>[12x]MERNHWNEKSSGAKRSRERDLTLSTIRSILAADERLRIKASSYLGVGRGVDDEAVIDIFPTGQTMSFLRLLHGFLGTCRGQSMHQVLRDPCVLRKQLLYGVCKTLFDTITVRRVAEEWKLHAALFPYRALDEEDLEQYLLVWSASLRQSVQTGVLGALRDILYQYADNDDYGLYVDWCVTVGLVPLLDVKTKPSEAAERAQFVRAAVQRATETHPLAQDLLQANLALLLQVAERLGAVRVANAPEVRVFKKVRSERLEAQLRGKHIRLYVAAEPLAYERDKLLFTTPVAHLHEEILRYDGLCRHQKICQLLNTFPVKVVTASRHELNCKKLVEMMEQHDRGSDAKKSIM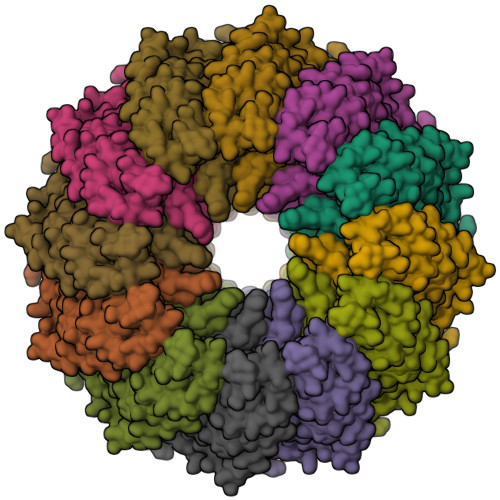KFLLNVSDSKSRIGIEDSVESFLQDLTPSLVDQNRLLPARGPGGPGVVGPGGAVVGGPAGHVGLLPPPPGPAAPERDIRDLFKKQVIKCLEEQIQSQVDEIQDLRTLNQTWENRVRELRDLLTRYASRREDSMSLGARDAELYHLPVLEAVRKARDAAPFRPLAVEDNRLVANSFFSQFVPGTESLERFLTQLWENEYFRTFRLRRLVTHQGAEEAIVYSNYTVERVTLPYLCHILALGTLDPVPEAYLQLSFGEIVAAAYDDSKFCRYVELICSREKARRRQMSREAAGGVPERGTASSGGPGTLERSAPRRLITADEERRGPERVGRFRNGGPDDPRRAGGPYGFH> SNATIYRMVDLPVIQPRLCTHARWPAPVYGLLVDPSLPSNPQWQNGRVHVDGTLLGTTPISGSWVSCFAAEAAYEFQSGTGEVATFTLIEQDGSAYVPGDRAAPLGYPDFSGQLEIEVQTETTKTGDKLKVTTFEMILGPTTNADQAPYQGRVFASVTAAASLDLVDGRVRAVPRSIYGFQDTIPEYNDGLLVPLAPPIGPFLPGEVLLRFRTYMRQIDTADAAAEAIDCALPQEFVSWFASNAFTVQSEALLLRYRNTLTGQLLFECKLYN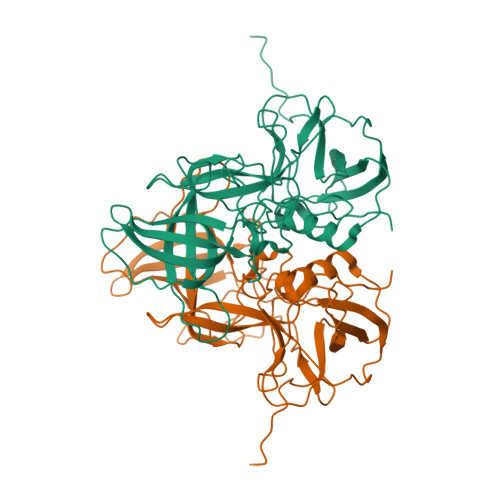EGYIALSYSGSGPLTFPTDGIFEVVSWVPRLYQLASVGSLATGRMLKQ>[4x]CTRFVYIGENNQVMTARSMDWKTDVGTNLWVFPRGMERSGEAGPNSVKWTSKYGSVIASGYDVSTTDGMNEAGLAANVLWLVESSYPDYDGKSPGL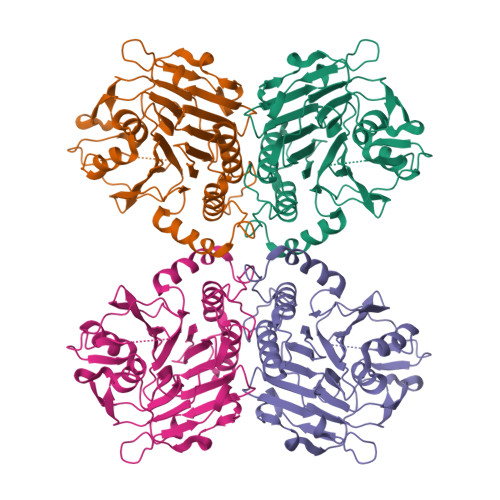SIAAWAQYVLDNFATVEEAVRVLEKNPFIIVTDSVPGEERLATLHLSLSDASGDSAIVEYIDGKQVIHHGRQYQVMTNSPTFDEQLALNAYWTQIGGTVMLPGTNRASDRFVRASFYANAIPKSENPVEAIASVFSVIRNVSVPYGITTPDQPNISSTRWRTVIDHKRKLYFFESALTPNVFWIDMTKLDLSKETGAVKKLDLGANQIHIYSGMANESLKDTKPFKFLGL> SNAVVEDSMKATSAEDLSNSIANQNPRGRGGDEDEELEEGEIVGDDDLDSSNLSASLVHQPHPLEHSWTFWFDNPSAKSKQATWGASIRPIYTFSTVEEFWSVYNNIHHPSKLAMRADLYCFKHKIEPKWEDPVCANGGKWTVNFPRGKSDNGWLYTLLAMIGEQFDCGDEICGAVVNVRSGQDKISIWTKNASNEAAQASIGK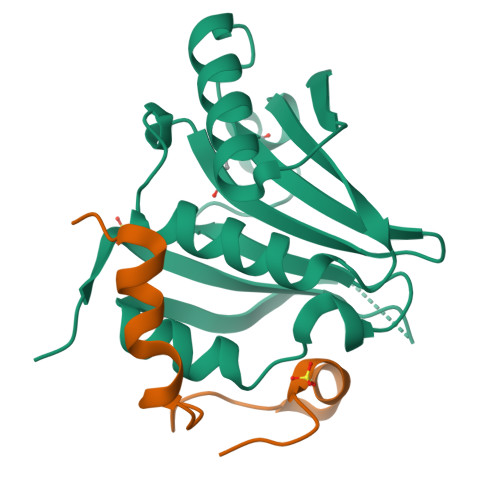QWKEFLDYNESIGFIFHDDAKKFDRHAKNKYMV;> NEAIKEDAGALSKAEPDDWEDAADIATPDLESANGDGVGTSMLDSGDRTGDMAKKYSRDFLLKFAEQFLDLPHNFEVTSDIESLMSTHTN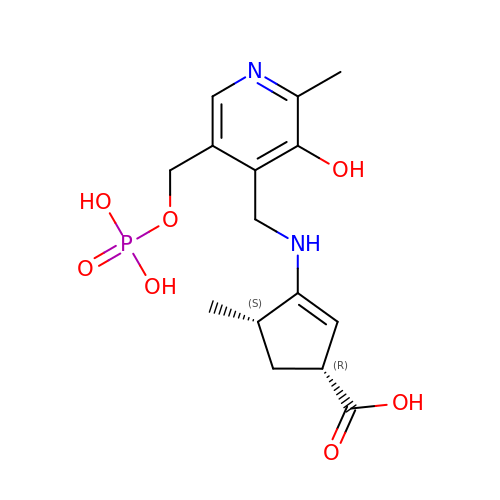(1~{R},3~{S},4~{R})-3-methyl-4-[[2-methyl-3-oxidanyl-5-(phosphonooxymethyl)pyridin-4-yl]methylamino]cyclopentane-1-carboxylic acid | C15 H21 N2 O7 P | LZIGREAGJMTTOE-WCBMZHEXSA-N3-{4-[(phenylcarbamoyl)amino]-1H-pyrazol-1-yl}-N-(3,4,5-trimethoxyphenyl)benzamide | C26 H25 N5 O5 | 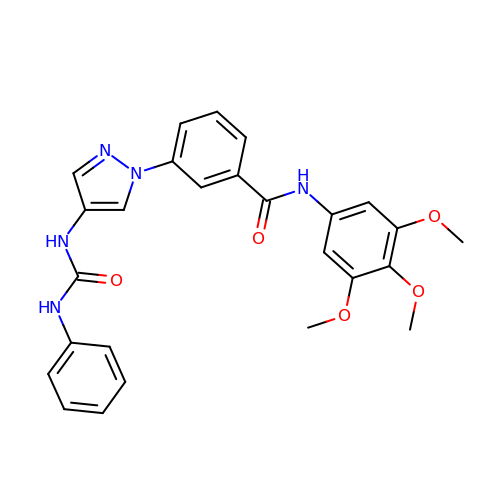RQEFLPVRZJPIAZ-UHFFFAOYSA-N>[6x]STFVAKDGTQIYFKDWGSGKPVLFSHGWLLDADMWEYQMEYLSSRGYRTIAFDRRGFGRSDQPWTGNDYDTFADDIAQLIEHLDLKEVTLVGFSMGGGDVARYIARHGSARVAGLVLLGAVTPLFGQKPDYPQGVPLDVFARFKTELLKD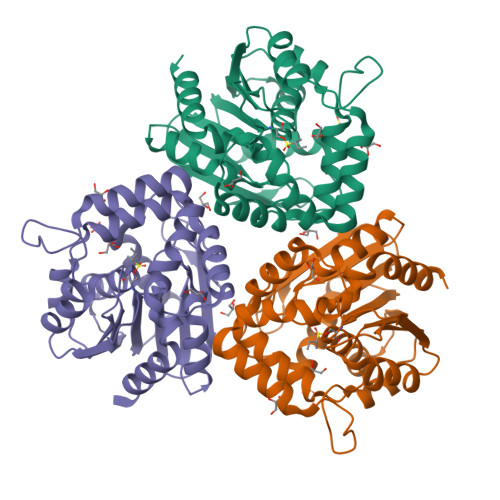RAQFISDFNAPFYGINKGQVVSQGVQTQTLQIALLASLKATVDCVTAFAETDFRPDMAKIDVPTLVIHGDGDQIVPFETTGKVAAELIKGAELKVYKDAPHGFAVTHAQQLNEDLLAFLKR> MCDLRKTKLIDKISSLELYKYSIFFRNYIENVAEDCLKNGLILESAAHNVSEVELARLKVQLKNALLNCIISYRFHGIGYVLVKTKDTLIDLEQPVNIELPIGFEYLDYEYVRDLGVDFDHITYKVKSNNKNNSLDAVKIHKSRLIIYENFDYILKRYVPCYTESFLLDIYLFEKIYVEIERRIENHNFLFYKDESLVQLQDALSSATTSLSALTQSNNDRGSGILSSFLRKQNSNNHSKDISNLRNLNDSLSQELARLKSNLNNEGMFYTATPSASLEVIKYDLSYLKEALALIKAKIGADTKEPLTRSFNEQAKGLGNDGKGDRSNYYDFLKGVQEQVENSCNLKLTKYFGLDMKFNSLIMLSEEQKVERDIKLIELYSKYNQLIQSSSFNNEELAMLKEKLF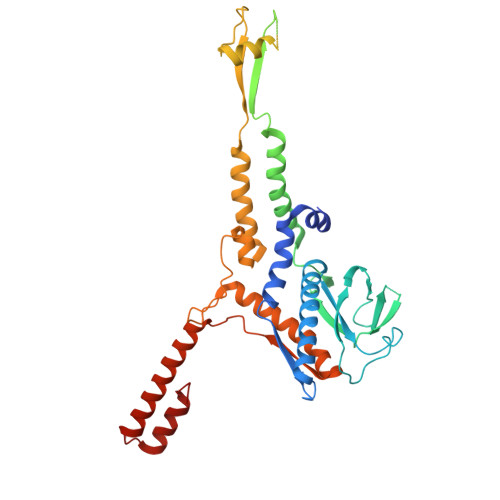SF(2S)-N,2-dicyclohexyl-2-[2-(5-phenylthiophen-2-yl)-1H-benzimidazol-1-yl]acetamide | C31 H35 N3 O 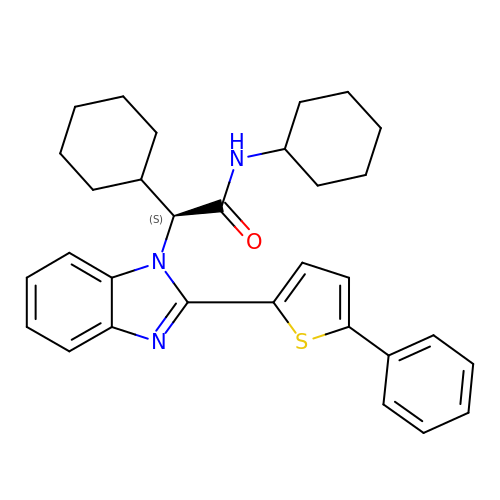S | AUFPVOAEDLSRHU-LJAQVGFWSA-N(2R,4R)-4-aminopyrrolidine-2,4-dicarboxylic 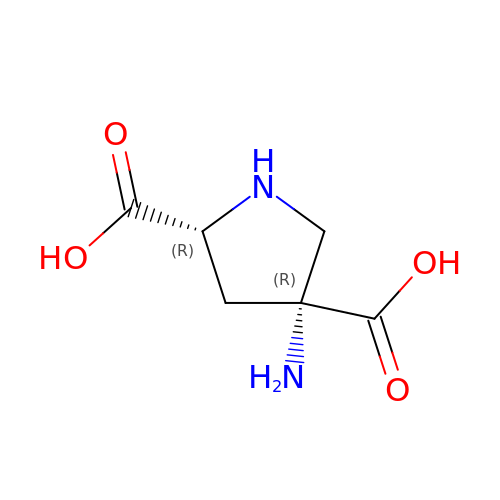acid | C6 H10 N2 O4 | XZFMJVJDSYRWDQ-AWFVSMACSA-N> MILIKLKVKGYITTQMRRIRNYYFSITNYIPSTTLRGAILAEYYNQTGKIDENFYVSPAYPIKTAPAHYFSPAKERKGDEFIEVKRILEKKEKEFEANKPIEEIMKLEIDGKHPKPKIGSLITYEGETDKENKYREFSSKSIIQMHVAIDKTSISSYKGMLFAYEYKEFDEMWAIASDSEVIDTVKRIKIGRGKNRGNKVVDVEKVREVSLDQSKGLLYCLSPCIGSLFGKTFFKAKYIIGDKSIYSGWFTVDSFSGQKPVFETLREGSLVYVESFSNEKSLMPAGLNFM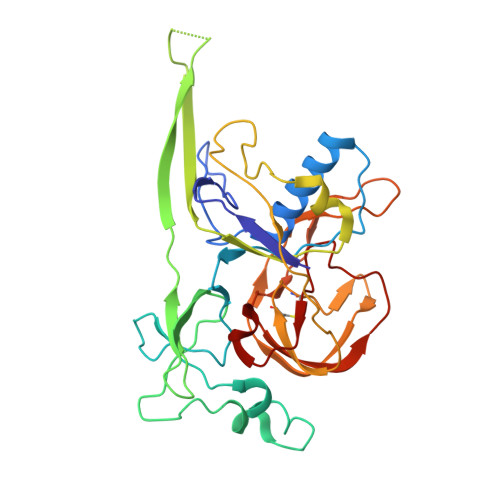LRISDLSSIL> SGISLDNSYKMDYPEMGLCIIINN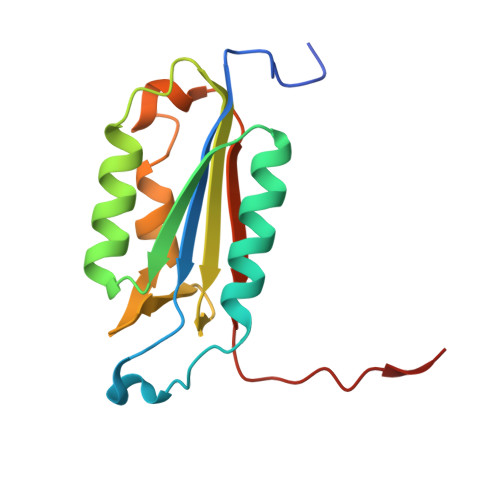KNFHKSTGMTSRSGTDVDAANLRETFRNLKYEVRNKNDLTREEIVELMRDVSKEDHSKRSSFVCVLLSHGEEGIIFGTNGPVDLKKITNFFRGDRCRSLTGKPKLFIIQACRGTEYDCGIETD>MFPTGWRPKLSESIAASRMLWQPMAAVAVVQIGLLWFSPPVWGQDMVSPPPPIA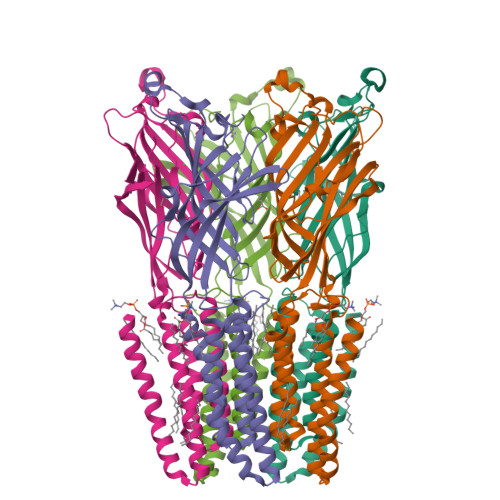DEPLTVNTGIYLIECYSLDDKAETFKVNAFLSLSWKDRRLAFDPVRSGVRVKTYEPEAIWIPEIRFVNVENARDADVVDISVSPDGTVQYLERFSARVLSPLDFRRYPFDSQTLHIYLIVRSVDTRNIVLAVDLEKVGKNDDVFLTGWDIESFTAVVKPANFALEDRLESKLDYQLRISRQYFSYIPNIILPMLFILFISWTAFWSTSYEANVTLVVSTLIAHIAFNILVETNLPKTPYMTYTGAIIFMIYLFYFVAVIEVTVQHYLKVESQPARAASITRASRIAFPVVFLLANIILAFLFFGF[5x]>AVSKVYARSVYDSRGNPTVEVELTTEKGVFRSIVPSGASTGVHEALEMRDGDKSKWMGKGVLHAVKNVNDVIAPAFVKANIDVKDQKAVDDFLISLDGTANKSKLGANAILGVSLAASRAAAAEKNVPLYKHLADLSKSKTSPYVLPVPFLNVLNGGSHAGGALALQEFMIAPTGAKTFAEALRIGSEVYHNLKSLTKKRYGASAGNVGDEGGVAPNIQTAEEALDLIVDAIKAAGHDGKVKIGLDCASSEFFKDGKYDLDFKNPNSDKSKWLTGPQLADLYHSLMKRYPIVSIEDPFAEDDWEAWSHFFKTAGIQIVADDLTVTNPKRIATAIEKKAADALLLKVNQIGTLSESIKAAQDSFAAGWGVMVSHRSGETEDTFIADLVVGLRTGQIKTGAPARSERLAKLNQLLRIEEELGDNAVFAGENFH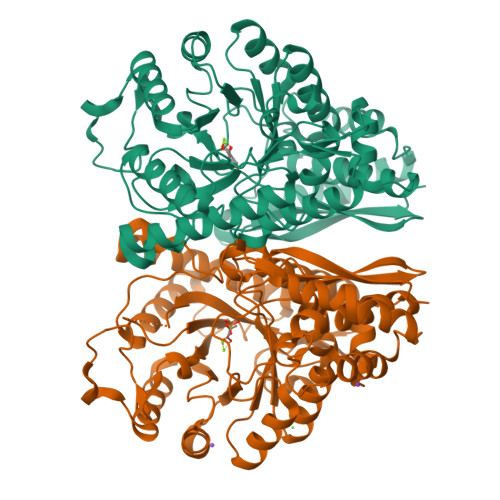HGDKL[2x]> GPGSHDLSKWKYAELRDTINTSC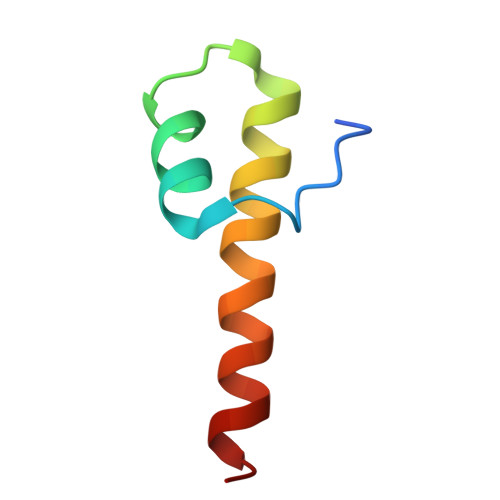DIELLAACREEFHRRLKVYHAWKSKN>QPITEEEQAAKLKAEKIRVALEKIKEAQVKKLVIRVHMSDDSSKTMMVDERQTVRQVLDNLMDKSHCGYSLDWSLVETVSELQMERIFEDHENLVENLLNWTRDSQNKLIFMERIEKYALFKNPQNYLLGKKETAEMADRNKEVLLEECFCGSSVTVPEIEGVLWLK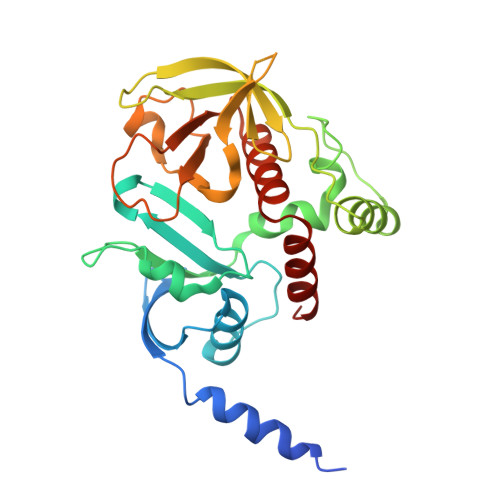DDGKKSWKKRYFLLRASGIYYVPKGKAKVSRDLVCFLQLDHVNVYYGQDYRNKYKAPTDYCLVLKHPQIQKKSQYIKYLCCDDVRTLHQWVNGIRIAKYGKQLYMNYQEALKRT[2x]>[2x]MKKLFLVFWWHMHQPLYREPYTGEYLLPWTFFHAVKDYYDMPAYLKDFEIKLNFNLTPVLIDQIQEYAQGKAKDVFLEAIRKDPDDLEKEEVEKLIEFTKLNYEKPIYRFERIRELMNKEKLNREELLDLQTLNLLAWCGRTLRKDLKDLLNK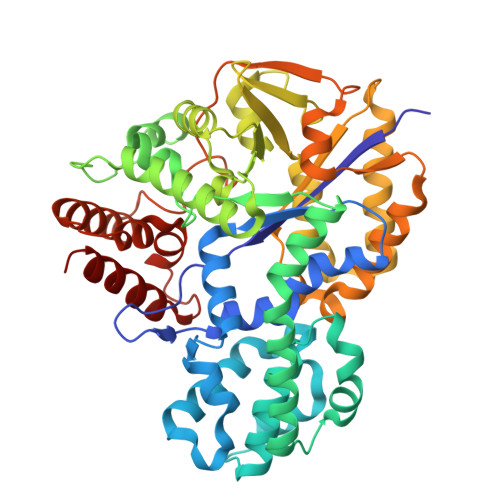GRNYTQEEKEYVLNKYFEIIKKTLSIYREIKEEGKGSVSTSPYYHPLIPILLNPNCVYETTPNVKIPDFAVSFREDASKHVELAKEKYFEIFGEHPVYMWPPEASVSNEALELYYEKGINMLATDEVILKNSVERASPYLRYYFRELISVFFRDKTLSDLIGFSYHAWNAEDAVRDFIGRLKKIHESVDFQPVVFVVLDGENCWEYYEENGIPFLEKLYSTLEKEEWIETLTLEEAMRKEDVKTEVIESVKAGTWFDGNFLKWIGNKEKNEYWKILIEAKKKAKNDYILVAEGSDWFWWQGEEKAPFVEVFDKLFRSFVRRAQE> MRGSHHHHHHGSMSETAKKVIVGMSGGVDSSVSAWLLQQQGYQVEGLFMKNWEEDDGEEYCTAAADLADAQAVCDKLGIELHTVNFAAEYWDNVFELFLAEYKAGRTPNPDILCNKEIKFKAFLEFAAEDLGADYIATGHYVRRADVDGKSRLLRGLDSNKDQSYFLYTLSHEQIAQSLFPVGELEKPQVRKIAEDLGLVTAKKKDSTGICFIGERKFREFLGRYLPAQPGKIITVDGDEIGEHQGLMYHTLGQRKGLGIGGTKEGTEEPWYVVDKDVENNILV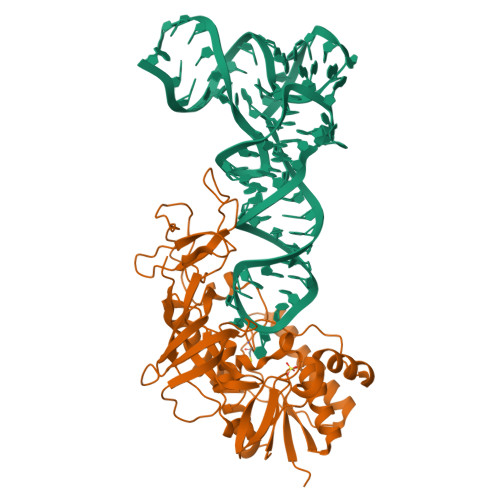VAQGHEHPRLMSVGLIAQQLHWVDREPFTGTMRCTVKTRYRQTDIPCTVKALDDDRIEVIFDEPVAAVTPGQSAVFYNGEVCLGGGIIEQRLPLPV> MNVTVDQSTLAGATRGIVRGGETLKEHRDRLMAATKATGRYAGLKTLELREREPILYNKLFSRLRAGVVDARETAKKIAASPIVEQEGELCFTLYNAAGDSLLTSTGIIIHVGTMGAAIKYMIENNWEANPGVHDKDIFCNNDSLIGNVHPCDIHTIVPIFWEGELIGWVGGVTHVIDTGAVGPGSMATGQVQRFGDGYSITCRKVGANDTLFRDWLHESQRMVRTTRYWMLDERTRIAGCHMIRKLVEEVVAEEGIEAYWKFAYEAVEHGRLGLQARIKAMTIPGTYRQVGFVDVPYAHEDVRVPSDFAKLDTIMHAPCEMTIRRDGTWRLDFEGSSRWGWHTYNAHQVSFTSGIWVMMTQTLIPSEMINDGAAYGTEFRLPKGTWMNPDDRRVAFSYSWHFLVSAWT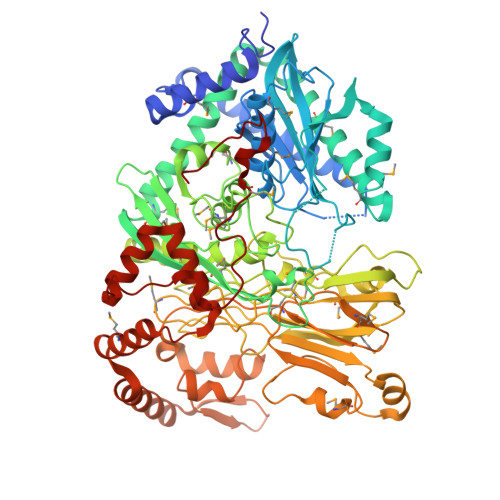ALWRGLSRSYFGRGYLEEVNAGNANTSNWLQGGGFNQYDEIHAVNSFECAANGTGATAVQDGLSHAAAIWNPEGDMGDMEIWELAEPLVYLGRQIKASSGGSGKYRGGCGFESLRMVWNAKDWTMFFMGNGHISSDWGLMGGYPAASGYRFAAHKTNLKELIASGAEIPLGGDTDPENPTWDAMLPDAQIKRDKQAITTEEMFSDYDLYLNYMRGGPGFGDPLDREPQAVADDINGGYVLERFAGEVYGVVVRKGADGQYGVDEAGTAAARAQIRKDRLAKSVPVSEWMKGEREKILAKDAGTQVRQMFAASFKLGPRFEKDFRTFWSLPDSWTLPEEEIGVPTYGSRYSMDISELPDVHTVQFVEE> AAAAAAAAAAAAAAAAAAAAAAAAAAAAAAAAAAAAAAAAAAAAAAAAAAAAAAAAAAAAAAAAAAAAAAAAAAAAAAAAAAAAAAAAAAAAAAAAAAAAAAAAAAAAAAAAAAAAAAAAAAAAAAAAAAAAAAAAAAAAAAAAAAAAAAAAAAAAAAAAAAAAAAAAAAAAAAAAAAAAAAAAAAAAAAAAAAAAAAAAAAAAAAAAAAAAAAAAAAAAAAAAAAAAAAAAAAAAAAAAAAAAAAAAAAAAAAAAAAAAAAAAAAAAAAAAAA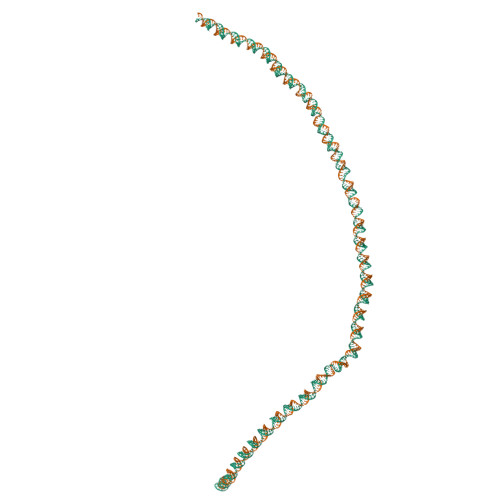AAAAAAAAAAAAAAAAAAAAAAAAAAAAAAAAAAAAAAAAAAAAAAAAAAAAAAAAAAAAAAAAAAAAAAAAAAAAAAAAAAAAAAAAAAAAAAAAAAAAAAAAAAAAAAAAAAAAAAAAAAAAAAAAAAAAAAAAAA;> AAAAAAAAAAAAAAAAAAAAAAAAAAAAAAAAAAAAAAAAAAAAAAAAAAAAAAAAAAAAAAAAAAAAAAAAAAAAAAAAAAAAAAAAAAAAAAAAAAAAAAAAAAAAAAAAAAAAAAAAAAAAAAAAAAAAAAAAAAAAAAAAAAAAAAAAAAAAAAAAAAAAAAAAAAAAAAAAAAAAAAAAAAAAAAAAAAAAAAAAAAAAAAAAAAAAAAAAAAAAAAAAAAAAAAAAAAAAAAAAAAAAAAAAAAAAAAAAAAAAAAAAAAAAAAAAAAAA;> AAAAAAAAAAAAAAAAAAAAAAAAAAAAAAAAAAAAAAAAAAAAAAAAAAAAAAAAAAAAAAAAAAAAAAAAAAAAAAAAAAAAAAAAAAAAAAAAAAAAAAAAAAAAAAAAAAAAAAAAAAAAAAAAAAAAAAAAAAAAAAAAAAAAAAAAAAAAAAAAAAAAAAAAAAAAAAAAAAAAAAAAAAAAAAAAAAAAAAAAAAAAAAAAAAAAAAAAAAAAAAAAAAAAAAAAAAAAAAAAAAAAAAAAAAAAAAAAAAAAAAAAA;> UUUUUUUUUUUUUUUUUUUUUUUUUUUUUUUUUUUUUUUUUUUUUUUUUUUUUUUUUUUUUUUUUUUUUUUUUUUUUUUUUUUUUUUUUUUUUUUUUUUUUUUUUUUUUUUUUUUUUUUUUUUUUUUUUUUUUUUUUUUUUUUUUUUUUUUUUUUUUUUUUUUUUUUUUUUUUUUUUUUUUUUUUUUUUUUUUUUUUUUUUUUUUUUUUUUUUUUUUUUUUUUUUUUUUUUUUUUUUUUUUUUUUUUUUUUUUUUUUUUUUUUUUUUUUUUUUUUUUUUUUUUUUUUUUUUUUUUUUUUUUUUUUUUUUUUUUUUUUUUUUUUUUUUUUUUUUUUUUUUUUUUUUUUUUUUUUUUUUUUUUUUUUUUUUUUUUUUUUUUUUUUUUUUUUUUUUUUUUUUUUUUUUUUUUUUU;> UUUUUUUUUUUUUUUUUUUUUUUUUUUUUUUUUUUUUUUUUUUUUUUUUUUUUUUUUUUUUUUUUUUUUUUUUUUUUUUUUUUUUUUUUUUUUUUUUUUUUUUUUUUUUUUUUUUUUUUUUUUUUUUUUUUUUUUUUUUUUUUUUUUUUUUUUUUUUUUUUUUUUUUUUUUUUUUUUUUUUUUUUUUUUUUUUUUUUUUUUUUUUUUUUUUUUUUUUUUUUUUUUUUUUUUUUUUUUUUUUUUUUUUUUUUUUUUUUUUUUUUUUUUUUUUUUUUU;> UUUUUUUUUUUUUUUUUUUUUUUUUUUUUUUUUUUUUUUUUUUUUUUUUUUUUUUUUUUUUUUUUUUUUUUUUUUUUUUUUUUUUUUUUUUUUUUUUUUUUUUUUUUUUUUUUUUUUUUUUUUUUUUUUUUUUUUUUUUUUUUUUUUUUUUUUUUUUUUUUUUUUUUUUUUUUUUUUUUUUUUUUUUUUUUUUUUUUUUUUUUUUUUUUUUUUUUUUUUUUUUUUUUUUUUUUUUUUUUUUUUUUUUUUUUUUUUUUUUUUUUUU>DISTVPDETYDALKLDRGKATPKETYEALVKRYKDPAHGAGKGTMGDYWEPIAISIYMDPNTFYKPPVSPKEVAERKDCVECHSDETPVWVRAWKRSTHANLDKIRNLKSDDPLYYKKGKLEEVENNLRSMGKLGEKETLKEVGCIDCHVDVNKKDKADHTKDIRMPTADTCGTCHLREFAERESERDTMVWPNGQWPAGRPSHALDYTANIETTVWATMPQREVAEGCTMCHTNQNKCDNCHTRHEFSAAESRKPEACATCHSGVDHNNWEAYTMSKHGKLAEMNRDKWNWEVRLKDAFSKGGQNAPTCAACHMEYEGEYTHNITRKTRWANYPFVPGIAENITSDWSEARLDSWVLTCTQCHSERFARSYLDLMDKGTLEGLAKYQEANAIVHKMYEDGTLTGQ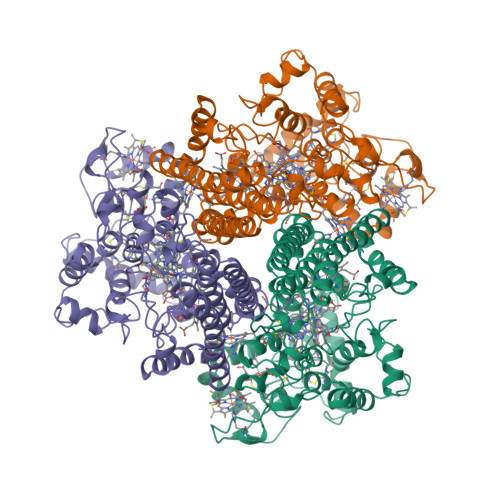KTNRPNPPEPEKPGFGIFTQLFWSKGNNPASLELKVLEMGENNLAKMHVGLAHVNPGGWTYTEGWGPMNRAYVEIQDEYTKMQELSALQARVNKLEGKQTSLLDLKGTGEKISLGGLGGGMLLAGALALIGWRKRKQTRA[2x]N-(1-CYANOCYCLOPROPYL)-3-({[(2S)-5-OXOPYRROLIDIN-2-YL]METHYL}SULFONYL)-N~2~-[(1S)-2,2,2-TRIFLUORO-1-(4-FLUOROPHENYL)ETHYL]-L-ALANINAMIDE 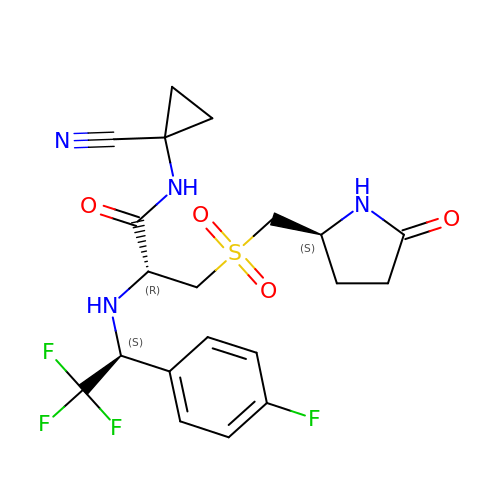| C20 H22 F4 N4 O4 S | JLPXDVXMMYRTKN-ZOBUZTSGSA-N> SKVMTLKDAIAKYVHSGDHIALGGFTTDRKPYAAVFEILRQGITDLTGLGGAAGGDWDMLIGNGRVKAYINCYTANSGVTNVSRRFRKWFEAGKLTMEDYSQDVIYMMWHAAALGLPFLPVTLMQGSGLTDEWGISKEVRKTLDKVPDDKFKYIDNPFKPGEKVVAVPVPQVDVAIIHAQQA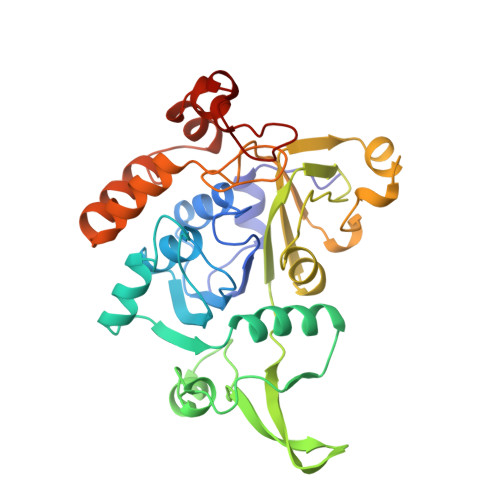SPDGTVRIWGGKFQDVDIAEAAKYTIVTCEEIISDEEIRRDPTKNDIPGMCVDAVVLAPYGAHPSQCYGLYDYDNPFLKVYDKVSKTQEDFDAFCKEWVFDLKDHDEYLNKLGATRLINLKVVPGLGYHIDMTKE The bifunctional enzyme Δ1-pyrroline-5-carboxylate synthase (P5CS) is vital to the synthesis of proline and ornithine, playing an essential role in human health and agriculture. The P5CS molecule contains two domains, GK and GPR, catalyzing the first and second steps in the biosynthesis of proline from glutamate. The GK domain catalyzes glutamate phosphorylation, and the GPR domain catalyzes the NADPH-dependent reduction of γ-glutamyl phosphate (G5P) to glutamate-γ-semialdehyde (GSA). Our results describe the assembly mechanism of P5CS filaments, in which the GK domain forms tetramer and the GPR domain forms dimer structure, and both domains form specific interaction interfaces.

We obtained a structure of the GK domain with the binding of glutamate in the P5CSGlu filament and a second structure of the GK domain with G5P-Mg-ADP in the P5CSMix filament. In contrast, G5P and ADP extend towards each other in the P5CSMix filament, and glutamate at the binding site is converted into the intermediate G5P. At ABD of the P5CSMix filament, the phosphate donor ATP becomes an ADP, associating with an Mg2+. In the P5CSMix filament, the same segment shifts away from the top of the binding pocket and forms an open loop, in which residue M213 interacts with G5P. The helix-helix structure (residues 105–113, 115–124) at region I of the P5CSGlu filament transforms into a helix-loop-helix structure (residues 105–119, 120–122, 123–128) in the P5CSMix filament. This helix-loop-helix structure is referred to as the ‘hook’ structure. The hook interaction forms strong contacts via hydrogen bonds (M119-R124, L121-M123) and salt bridges (E116-R124). The GK domain of each protomer rotates approximately 10° around its central axis, causing the horizontal compression of the GK domain dimer. By comparing the structures of the GK domain with various ligands, we demonstrate the conformational changes, which may be associated with phosphorylation of the substrate glutamate.

>MLQNSFKLAQSLRNGFYRNAWRAFSSHGPRQPLVSPERRLEKAHPTFTERSQLKYARRLVVKLGSAVITREDNHGLALGRLASIVEQVAECHLEGREVMMVTSGAVAFGKQKLAQELLMSLSMRETLNPKDSKEFDGATLEPRAAAAVGQSGLMSLYDAMFAQYGVKIAQVLVTKPDFYNEETRNNLFCTLSELISLNIVPIINTNDAVSPPMFIRDDEPAGGARRGIPIKDNDSLSAMLAAEVQADLLILMSDVDGIYNKPPWEDGAKLMHTYTSDDSNSIEFGKKSKVGTGGMDSKVKAATWALDRGVSVVICNGMQEKAIKTIIGGRKVGTFFTEATESANAVPVEVMAENARTGSRQMQALTPAQRASAVNTLADLLVSREKFILDANAKDLAEAQKSGLAKPLLSRLSLNPAKLKNLSVGLKQIAEDSHKNVGRVLRRTRLADQLELKQVTVPIGVLLVIFESRPDSLPQVAALAMASANGLLLKGGKEAAHSNKALMELVKEALATVGAEHAVSLVSTREEISDLLSMENHIDLIIPRGSSDLVRSIQQQSLHIPVLGHAEGVCHVYIDRDADLEKALRIARDAKCDYPAACNAMETLLIHEDLMSGAIFGDVCNMLKREGVKIYAGPRLNQQLTFGPPAAKSLKHEYGALECCIEVVPSLDEAINHIHTYGSSHTDVIVTENDAAARQFLGSVDSACVFHNASSRFADGFRFGLGAEVGISTARIHARGPVGVEGLLTTKWILEGQDHAAADFAEGGGRTWLHETLPLD[8x]>[2x]SLENIMTLPKIKHVRAWFIGGATAEKGAGGGDYHDQGGNHWIDDHIATPMSKYRDYEQSRQSFGINVLGTLIVEVEAENRQTGFAVSTAGEMGCFIVEKHLN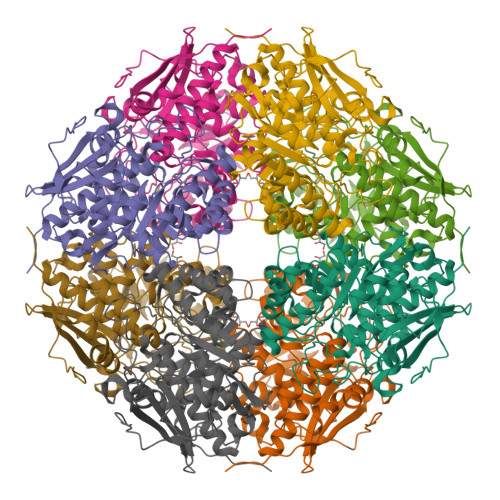RFIEGKCVSDIKLIHDQMLGATMYYSGSGGLVMNTISCVDLALWDLFGKVVGLPVYKLLGGAVRDEIQFYATGARPDLAKEMGFIGGKMPTHWGPHDGDAGIRKDAAMVADMREKCGPDFWLMLDCWMSQDVNYATKLAHACAPFNLKWIEECLPPQQYEGYRELKRNAPAGMMVTSGEHHGTLQSFRTLAETGIDIMQPDVGWCGGLTTLVEIAALAKSRGQLVVPHGSSVYSHHAVITFTNTPFSEFLMTSPDCSTLRPQFDPILLDEPVPVNGRIHKSVLDKPGFGVELNRDCHLKRPYSHEGHHHHHH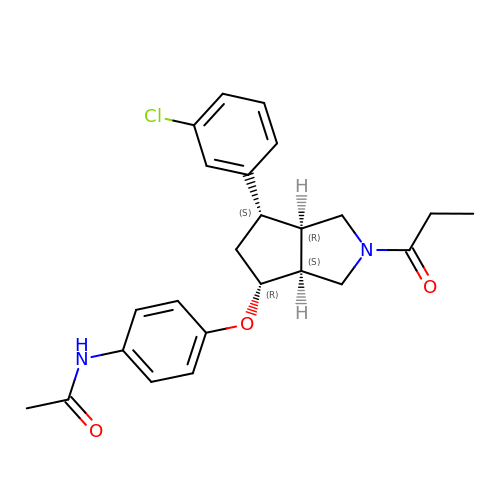N-(4-{[(3aS,4R,6S,6aR)-6-(3-chlorophenyl)-2-propanoyloctahydrocyclopenta[c]pyrrol-4-yl]oxy}phenyl)acetamide | C24 H27 Cl N2 O3 | BEXJJYBHLWEKDU-SSGKUCQKSA-N> MNDIIINKIATIKRCIKRIQQVYGDGSQFKQDFTLQDSVILNLQRCCEACIDIANHINRQQQLGIPQSSRDSFTLLAQNNLITQPLSDNLKKMVGLRNIAVHDYQELNLDIVVHVVQHHLEDFEQFIDV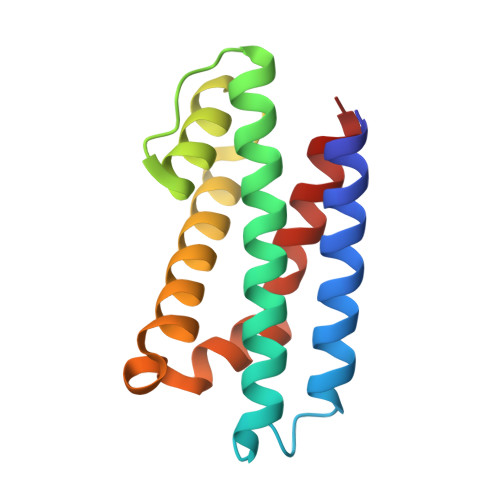IKAE> STTVHFEIGSIVGILITFINGPTEVYGQFLDGSPPLVWDKKDVPENKRTFKSKPRLLDIVLALYSDGCFYRAQIIDEFPSEYMI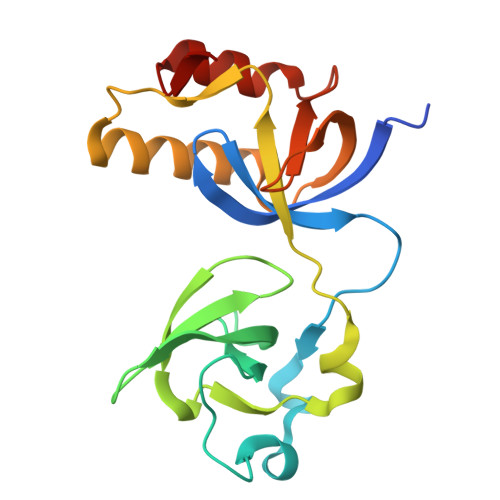FYVDYGNTEFVPLSCLAPCENVDSFKPHRVFSFHIEGIVRSKNLTHQKTIECIEYLKSKLLNTEMNVHLVQRLPDGFLIRFLDDWKYIPEQLLQRNYAQVSQ> GSSHHHHHHSSGLVPRGSMSTSWSDRLQNAADMPANMDKHALKKYRREAYHRVFVNRSLAMEKIKCFGFNMDYTLAVYKSPEYESLGFELTVERLVSIGYPQELLSFAYDSTFPTRGLVFDTLYGNLLKVDAYGNLLVCAHGFNFIRGPETREQYPNKFIQRDDTERFYILNTLFNLPETYLLACLVDFFTNCPRYTSCETGFKDGDLFMSYRSMFQDVRDAVDWVHYKGSLKEKTVENLEKYVVKDGKLPLLLSRMKEVGKVFLATNSDYKYTDKIMTYLFDFPHGPKPGSSHRPWQSYFDLILVDARKPLFFGE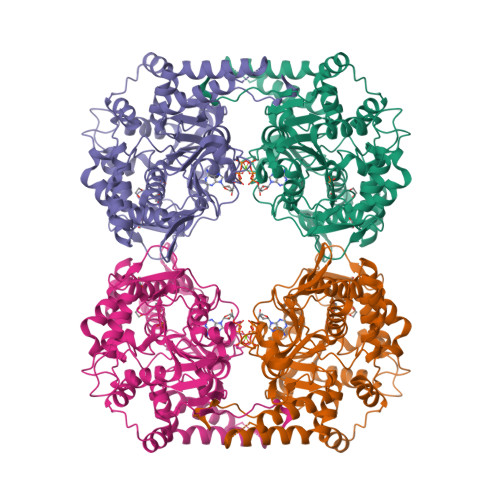GTVLRQVDTKTGKLKIGTYTGPLQHGIVYSGGSSDTICDLLGAKGKDILYIGDHIFGDILKSKKRQGWRTFLVIPEFAQELHVWTDKSSLFEELQSLDIFLAELYKHLDSSSNERPDISSIQRRIKKVTHDMDMCYGMMGSLFRSGSRQTLFASQVMRYADLYAASFINLLYYPFSYLFRAAHVLMPHESTVEHTHVDINEMESPLATRNRTSVDFKDTDYKRHQLTRSISEIKPPNLFPLAPQEITHCHDEDDDEEEEEEEE> METLGGFPVEFLIQVTR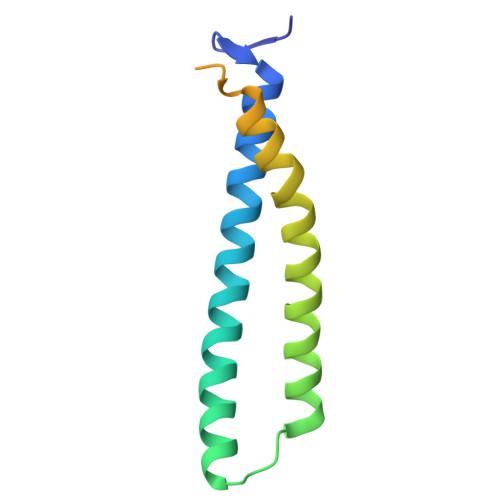LSKILMIKKEHIKKLREMNTEAEKLKSYSMPISIEFQRRYATIVLELEQLNKDLNKVLHKVQQYCYELAPDQGLQPADQPTDMRRRCEEEAQEIVRHANSST>[2x]MTKPLDGINVLDFTHVQAGPACTQMMGFLGANVIKIERRGSGDM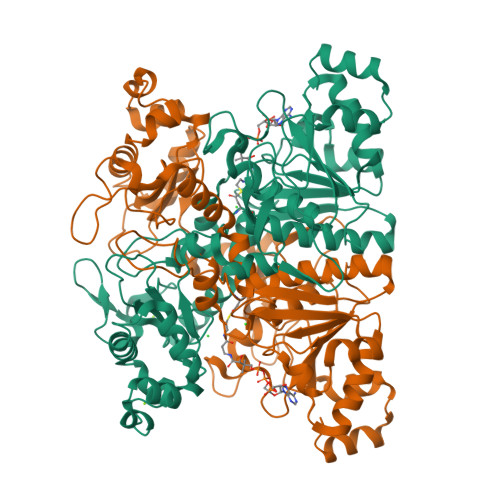TRGWLQDKPNVDSLYFTMFNCNKRSIELDMKTPEGKELLEQMIKKADVMVENFGPGALDRMGFTWEYIQELNPRVILASVKGYAEGHANEHLKVYENVAQCSGGAAATTGFWDGPPTVSGAALGDSNSGMHLMIGILAALEIRHKTGRGQKVAVAMQDAVLNLVRIKLRDQQRLERTGILAEYPQAQPNFAFDRDGNPLSFDNITSVPRGGNAGGGGQPGWMLKCKGWETDADSYVYFTIAANMWPQICDMIDKPEWKDDPAYNTFEGRVDKLMDIFSFIETKFADKDKFEVTEWAAQYGIPCGPVMSMKELAHDPSLQKVGTVVEVVDEIRGNHLTVGAPFKFSGFQPEITRAPLLGEHTDEVLKELGLDDAKIKELHAKQVV>APTSSSTKKTQLQL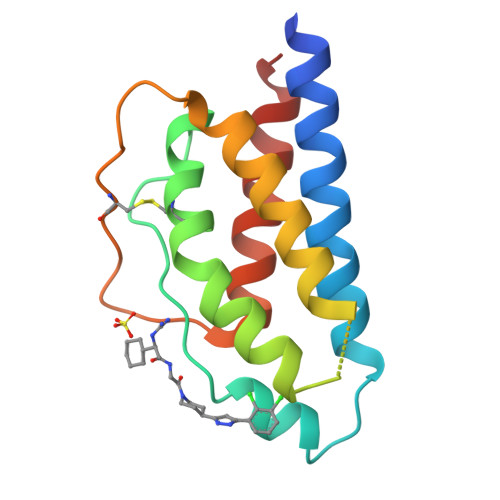EHLLLDLQMILNGINNYKNPKLTRMLTFKFYMPKKATELKHLQCLEEELKPLEEVLNLAQSKNFHLRPRDLISNINVIVLELKGSETTFMCEYADETATIVEFLNRWITFCQSIISTLT[2x]P1-(5'-ADENOSYL)-P5-(5'-GUANOSYL) PENTAPHOSPHATE | C20 H29 N10 O23 P5 | 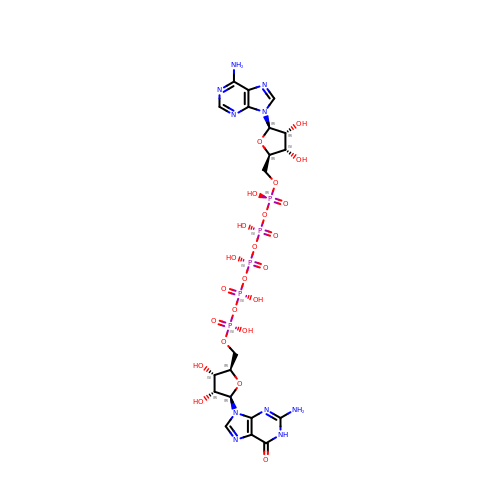CNMILLPGDWDFCZ-INFSMZHSSA-N> MEQNPQSQLKLLVTRGKEQGYLTYAEVNDHLPEDIVDSDQIEDIIQMINDMGIQVMEEAPDADDLMLAENTADEDAAEAAAQVLSSVESEIGRTTDPVRMYMREMGTVELLTREGEIDIAKRIEDGINQVQCSVAEYPEAITYLLEQYDRVEAEEARLSDLITGFVDPNAEEDLAPTATHVGSELSQEDLDDDEDEDEEDGDDDSADDDNSIDPELAREKFAELRAQYVVTRDTIKAKGRSHATAQEEILKLSEVFKQFRLVPKQFDYLVNSMRVMMDRVRTQERLIMKLCVEQCKMPKKNFITLFTGNETSDTWFNAAIAMNKPWSEKLHDVSEEVHRALQKLQQIEEETGLTIEQVKDINRRMSIGEAKARRAKKEMVEANLRLVISIAKKYTNRGLQFLDLIQEGNIGLMKAVDKFEYRRGYKFSTYATWWIRQAITRSIADQARTIRIPVHMIETINKLNRISRQMLQEMGREPTPEELAERMLMPEDKIRKVLKIAKEPISMETPIGDDEDSHLGD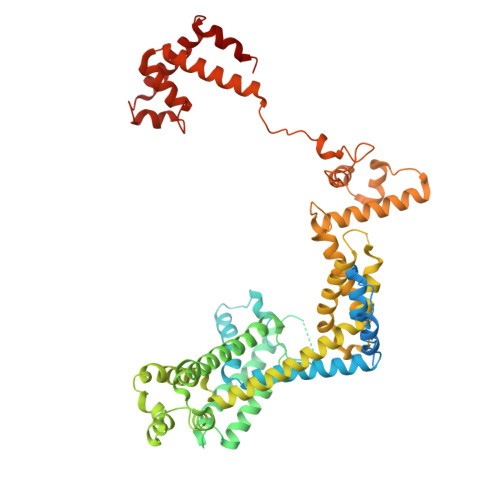FIEDTTLELPLDSATTESLRAATHDVLAGLTAREAKVLRMRFGIDMNTDYTLEEVGKQFDVTRERIRQIEAKALRKLRHPSRSEVLRSFLDD>[8x]MDKFRMMFQFLQSNQESFMNGICGIMALASAQMYSSFEFSCPCMPEYNYTYGIGLLIIPPIWFFLLGFVLNNNVSVLAEEWKRPTGRRTKDPSVLRYMLCSITQRSLIAPAVWVSVTLMDGKSFLCAFSINLDIEKFGNASLVIGMTETEKL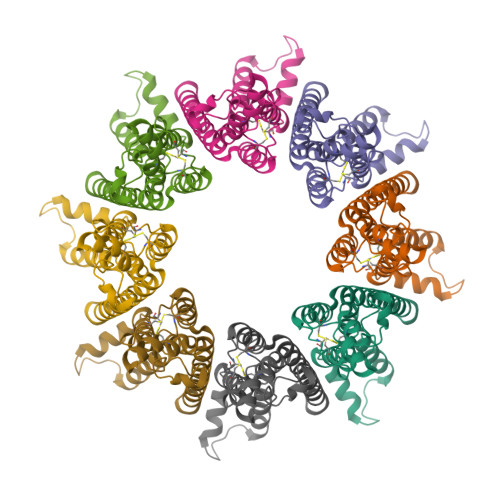KFLARIPCKDLFEDNEVRVAATRYIKCISQACGWMFLLMMTFTAFLIRAIRPCFTQASYRQEAYWAQYRANEDQLFQRTAEVHSRVLAANNVRRFFGFVALNKDDEELIANFPVEGTQPRPQWNAITGVYLYRENQGLPLYSRLHKWAQGLAGNGAAPDNVEMALLPSENLYFQ> TDSFLLRFLRARDFDLDLAWRLLKNYYKWRAECPEISADLHPRSIIGLLKAGYHGVLRSRDPTGSKVLIYRIAHWDPKVFTAYDVFRVSLITSELIVQEVETQRNGIKLIFDLEGWQFSHAFQITPSVAKKI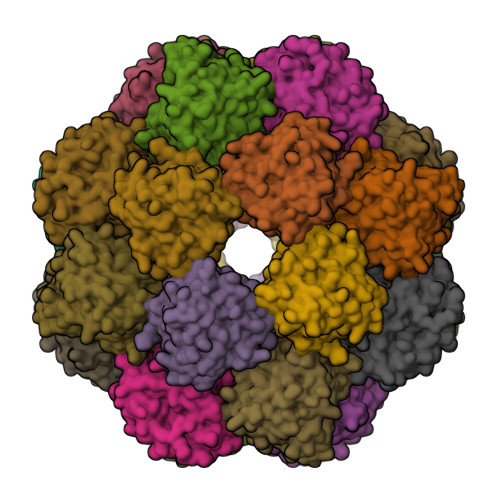AAVLTDSFPLKVRGIHLINEPVIFHAVFSMIKPFLTEKIKERIHMHGNNYKQSLLQHFPDILPLEYGGEEFSMEDICQEWTNFIMKSEDYLSSISESIQ>MKDILEKLEERRAQARLGGGEKRLEAQHKRGKLTARERIELLLDHGSFEEFDMFVQHRSTDFGMEKQKIPGDGVVTGWGTVNGRTVFLFSKDFTVFGGSLSEAHAAKIVKVQDMALKMRAPIIGIFDAGGARIQEGVAALGGYGEVFRRNVAASGVIPQISVIMGPCAGGDVYSPAMTDFIFMVRDTSYMFVTGPDVVKTVTNEVVTAEELGGAKVHTSKSSIADGSFENDVEAILQIRRLLDFLPANNIEGVPEIESFDDVNRLDKSLDTLIPDNPNKPYDMGELIRRVVDEGDFFEIQAAYARNIITGFGRVEGRTVGFVANQPLVLAGVLDSDASRKAARFVRFCNAFSIPIVTFVDVPGFLPGTAQEYGGLIKHGAKLLFAYSQATVPLVTIITRKAFGGAYDVMASKHVG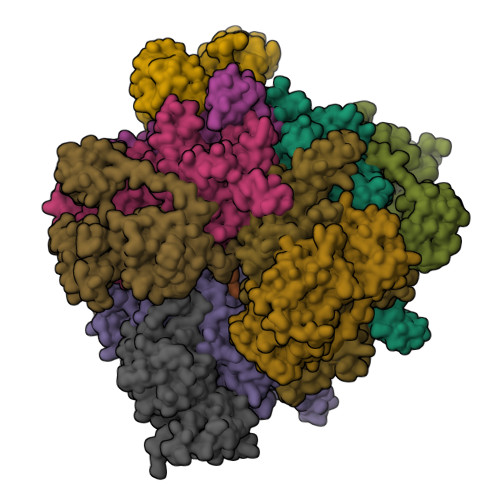ADLNYAWPTAQIAVMGAKGAVEIIFRAEIGDADKIAERTKEYEDRFLSPFVAAERGYIDEVIMPHSTRKRIARALGMLRTKEMEQPWKKHDNIPL[6x];>MFDKILIANRGEIACRIIKTAQKMGIKTVAVYSDADRDAVHVAMADEAVHIGPAPAAQSYLLIEKIIDACKQTGAQAVHPGYGFLSERESFPKALAEAGIVFIGPNPGAIAAMGDKIESKKAAAAAEVSTVPGFLGVIESPEHAVTIADEIGYPVMIKASAGGGGKGMRIAESADEVAEGFARAKSEASSSFGDDRVFVEKFITDPRHIEIQVIGDKHGNVIYLGERECSIQRRNQKVIEEAPSPLLDEETRRKMGEQAVALAKAVNYDSAGTVEFVAGQDKSFYFLEMNTRLQVEHPVTEMITGLDLVELMIRVAAGEKLPLSQDQVKLDGWAVESRVYAEDPTRNFLPSIGRLTTYQPPEEGPLGGAIVRNDTGVEEGGEIAIHYDPMIAKLVTWAPTRLEAIEAQATALDAFAIEGIRHNIPFLATLMAHPRWRDGRLSTGFIKEEFPEGFIAPEPEGPVAHRLAAVAAAIDHKLNIRKRGISGQMRDPSLLTFQRERVVVLSGQRFNVTVDPDGDDLLVTFDDGTTAPVRSAWRPGAPVWSGTVGDQSVAIQVRPLLNGVFLQHAGAAAEARVFTRREAELADLMPVKENAGSGKQLLCPMPGLVKQIMVSEGQEVKNGEPLAIVEAMKMENVLRAERDGTISKIAAKEGDSLAVDAVILEFA[6x]>[4x]MSIKVCIADDNRELVSLLDEYISSQPDMEVIGTAYNGQDCLQMLEEKRPDILLLDIIMPHLDGLAV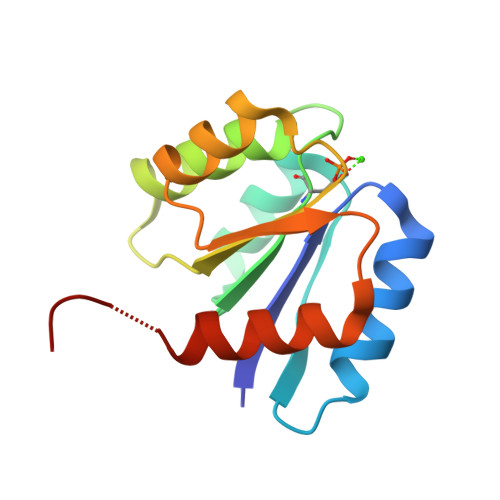LERIRAGFEHQPNVIMLTAFGQEDVTKKAVELGASYFILKPFDMENLAHHIRQVYGKTTPVVRK>[2x]MDWVVAPISVPENGKGPFPQRLVQLKSNKDRDTKIFYSITGPGADSPPEGVFAVEKETGWLLLNKP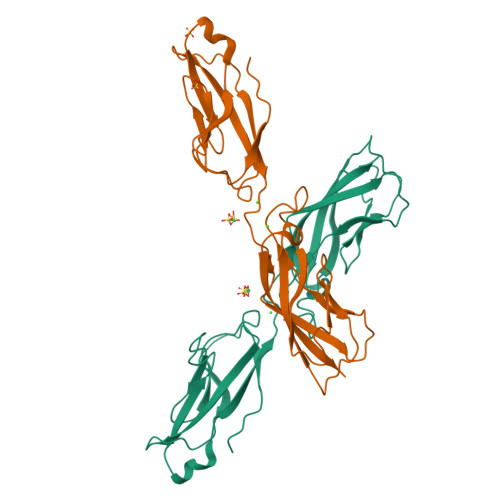LDREEIAKYELFGHAVSENGASVEDPMNISIIVTDQNDHKPKFTQDTFRGSVLEGVLPGTSVMQVTATDEDDAIYTYNGVVAYSIHSQEPKDPHDLMFTIHRSTGTISVISSGLDREKVPEYTLTIQATDMDGDGSTTTAVAVVEILD>MSGFKFLFFSPDGTLYGVHNDKLYKGTPPTSDNDNWLARATLIGN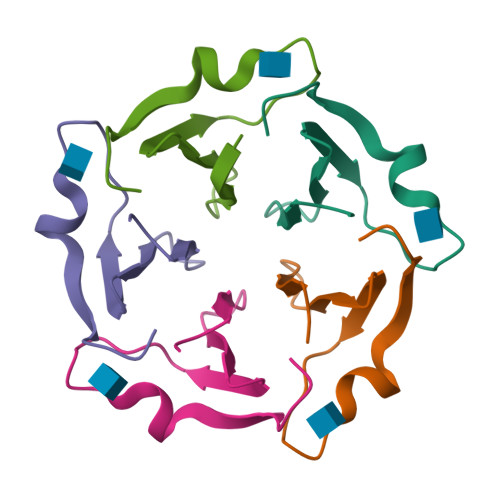GGW[15x]>CACGT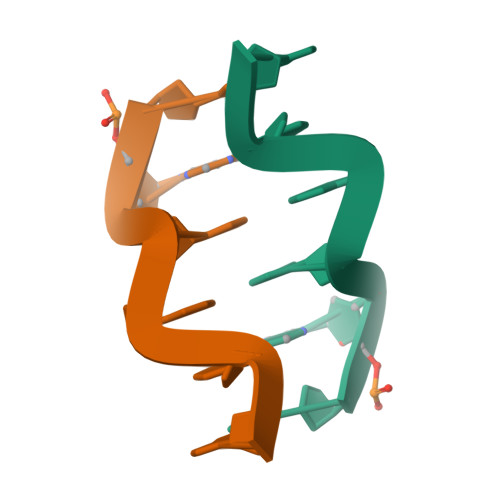G[2x]>[2x]MNSELDYYEKFEEVHGILMYKDFVKYWDNVEAFQARPDDLVIATYPKSGTTWVSEIVYMIYKEGDVEKCKEDVIFNRIPFLECRKENLMNGVKQLDEMNSPRIVKTHLPPELLPAS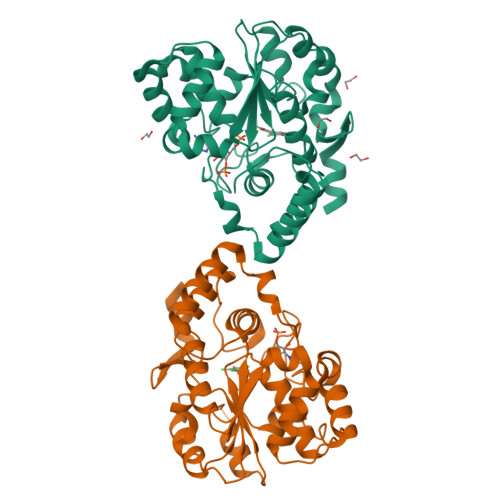FWEKDCKIIYLCRNAKDVAVSFYYFFLMVAGHPNPGSFPEFVEKFMQGQVPYGSWYKHVKSWWEKGKSPRVLFLFYEDLKEDIRKEVIKLIHFLERKPSEELVDRIIHHTSFQEMKNNPSTNYTTLPDEIMNQKLSPFMRKGITGDWKNHFTVALNEKFDKHYEQQMKESTLKFRTEI6-{[(3R,4R)-4-{[5-(6-aminopyridin-2-yl)pentyl]oxy}pyrrolidin-3-yl]methyl}-4-methylpyridin-2-amine 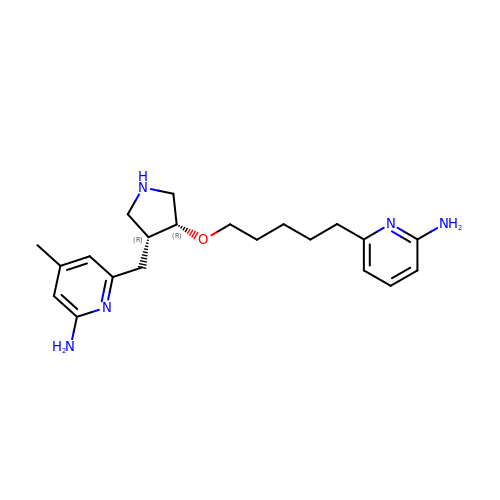| C21 H31 N5 O | ISEYRPTZYRJQPZ-APWZRJJASA-N> MSRKRSTKPKPAAKIALKKENDQFLEALKLYEGKQYKKSLKLLDAILKKDGSHVDSLALKGLDLYSVGEKDDAASYVANAIRKIEGASASPICCHVLGIYMRNTKEYKESIKWFTAALNNGSTNKQIYRDLATLQSQIGDFKSALVSRKKYWEAFLGYRANWTSLAVAQDVNGERQQAINTLSQFEKLAEGKISDSEKYEHSECLMYKNDVMYKAASDNQDKLQNVLKHLNDIEPCVFDKFGLLERKATIYMKLGQLKDASIVYRTLIKRNPDNFKYYKLLEVSLGIQGDNKLKKALYGKLEQFYPRCEPPKFIPLTFLQDKEELSKKLREYVLPQLKRGVPATFSNVKPLYQRRKSKVSPLLEKIVLDYLSGLDPTQDPIPFIWTNYYLSQHFLFLKDFPKAQEYIDAALDHTPTLVEFYILKARI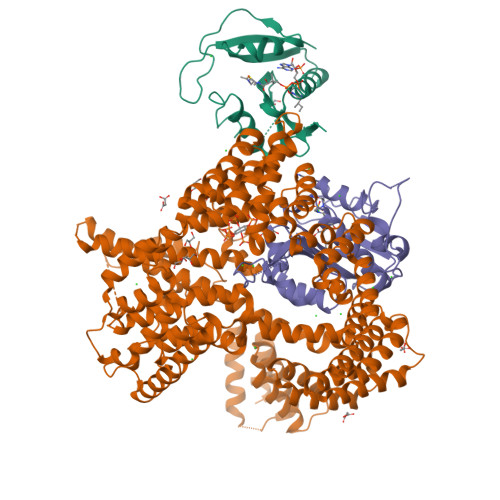LKHLGLMDTAAGILEEGRQLDLQDRFINCKTVKYFLRANNIDKAVEVASLFTKNDDSVNGIKDLHLVEASWFIVEQAEAYYRLYLDRKKKLDDLESLKKEVESDKSEQIANDIKENQWLVRKYKGLALKRFNAIPKFYKQFEDDQLDFHSYCMRKGTPRAYLEMLEWGKALYTKPMYVRAMKEASKLYFQMHDDRLKRKSDSLDENSDEIQNNGQNSSSQKKKAKKEAAAMNKRKETEAKSVAAYPSDQDNDVFGEKLIETSTPMEDFATEFYNNYSMQVREDERDYILDFEFNYRIGKLALCFASLNKFAKRFGTTSGLFGSMAIVLLHATRNDTPFDPILKKVVTKSLEKEYSENFPLNEISNNSFDWLNFYQEKFGKNDINGLLFLYRYRDDVPIGSSNLKEMIISSLSPLEPHSQNEILQYYL;> MPINIRRATINDIICMQNANLHNLPENYMMKYYMYHILSWPEASFVATTTTLDCEDSDEQDENDKLELTLDGTNDGRTIKLDPTYLAPGEKLVGYVLVKMNDDPDQQNEPPNGHITSLSVMRTYRRMGIAENLMRQALFALREVHQAEYVSLHVRQSNRAALHLYRDTLAFEVLSIEKSYYQDGEDAYAMKKVLKLEELQISNFTHRRLKENEEKLEDDLESDLLEDIIKQGVNDIIV;> MGRDICTLDNVYANNLGMLTKLAHVTVPNLYQDAFFSALFAEDSLVAKNKKPSSKKDVHFTQMAYYSEIPVGGLVAKLVPKKQNELSLKGIQIEFLGVLPNYRHKSIGSKLLKFAEDKCSECHQHNVFVYLPAVDDLTKQWFIAHGFEQVGETVNNFIKGVNGDEQDAILLKKHIS> MPFMWRQRAYCAPVPSAF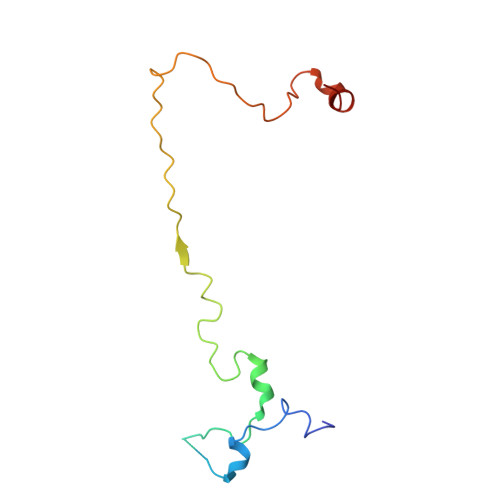ASQQPNGLGGEAGVRKPLLRSNSESLSVFSQIPDGLLGHTTSVTMGNSDIFFLPKPSNLLKIALPAFVFMPNLTIFTRAFPFYAHTSA> GIPAELRPGTNQFLTTDDGTAAPILPGFTPTPTIHIPGEVHSLLELCRVETILEVNNTTEATGLTRLLIPVSSQNKADELCAAFMVDPGRIGPWQSTLVGQICRYYTQ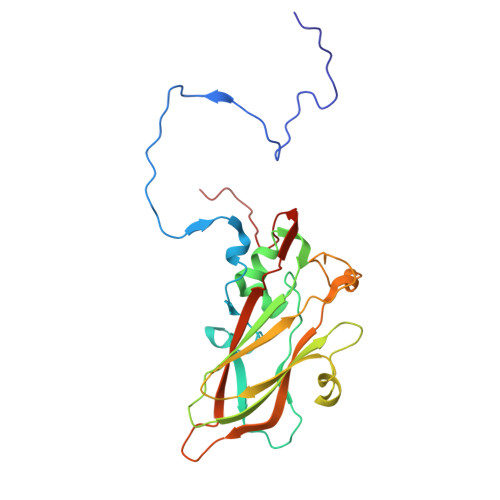WSGSLKVTFMFTGSFMATGKMLVAYSPPGSAQPANRETAMLGTHVIWDFGLQSSVSLVIPWISNTHFRTAKTGGNYDYYTAGVVTLWYQTNYVVPPETPGEAYIIAMGAAQDNFTLKICKDTDEVTQQAVLQ> GSGSPLAQQIKNTLTFIGQANAAGRM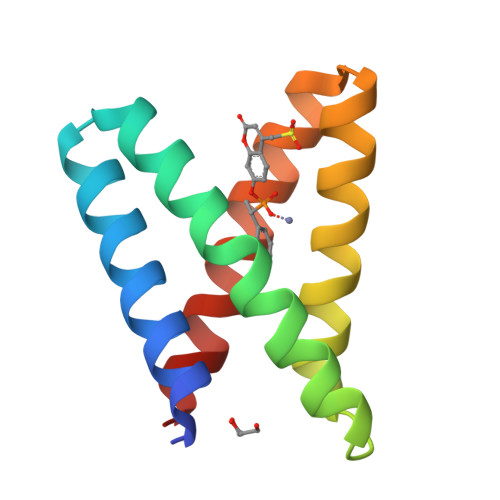DEVRTLQQNLHPLWAEYFQQTEGSGGSPLAQQIQYGHVLIHQARAAGRMDEVRRLSENTLQLMKEYFQQSD> MNKSQDEVKEDYFSIKKKKYNSLDCVLSPIVTRKKQESINSFQAGLQEDQNSTAVPESPFIRNCSETLNRSQHKILDHYFEYDYSLKKKIEKIKISLQNKTGTDSSQSLVQKRLDDLRKKTLIYKQFNIQKNNNNINNTGQFFIEKDKQNNLNLSQPHQIIKSKQGHKRSFTNTLYCSSNDKKIFNISSQKQNIKTVKQSNNSSMYEEQIKNDQNKKQNFNKQAKSERKQAEFCDLFYESMQKDAERQFKSNSDKSKSITQILENNCENAIVLLNHLIQILTDSIPISKNSILLDEKLSQCVNLSNNSKISQLMLVIQKLQGKISYYYNDFLKCIRMMKICKNFCQLFGTLKFKISCYKYIGLGFQRLNKPKVALVYFVKMLRQSWFLKQEDQEINSYDFIGMSYFYLGSIDKAYQYHQMMIDGIKADEEVKKISNIMLKNRKYSNYPTLQNIRIIQETSDGQPLQKTIRKSKIINPQFQLTQQEWGENISSSEDEFELPQMQIAVKNAEEQTFQKKFLSTPWNDRFIQAQIHKLEIAQELNYNKFPIGLVFKNQSVLNFPNSSNQPQLVVGPYANKIYNQELSSTYSSRQRISHQTPNREFFNYHSQLQQVKEQTQLNQMKQQYNQIVDSIELANHLIVLKNLKKVKDLFQNLIPYLNEKYYNIKQQNTKSLKQQQNSFDAQNSNQSFLGLQNYSIQINGILNINNQTDEYVNNQSDRSYQQQSDKLKLLIKSKSRNHSKEINMTQNYFKSPSNESKQIKNLRVIVDNSNKKKAQQKLNQEFSMNFCESPKYDNSILSLFINKLSQESALRLEIRQIGSASRYQRKKQQKGKQRKEKYQKKQEENKLNIKQYKKERYNMALFFMANTAIS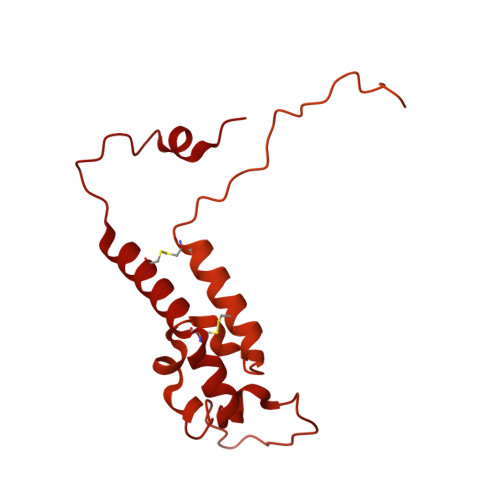VPSVLDTSPCMKQMLAYEDCVLDANVPQQEVIHPQWPTIWPRLLTDGKLLEFDKVPFHPENIYNYTYMRPLTKKNKQYLYECEEERFVFKACLRKVISLKKTDKHTSWDTAEVANLQLT Farnesyl pyrophosphate synthase (FPPS; EC 2.5.1.10) is a promising antibiotic drug target as it represents the point of convergence of these two pathways. The enzyme belongs to a large group of prenyltransferases responsible for the principal bond-forming reactions of isoprenoid biosynthesis. The mevalonate and nonmevalonate pathways both produce isopentenyl pyrophosphate (IPP), which along with its isomer dimethyl­allyl diphosphate (DMAPP) is converted through a ‘head-to-tail’ condensation reaction to form geranyl diphosphate (GPP) by FPPS. In summary, this work provides the first functional and structural insights into FPPS from the opportunistic pathogen P. aeruginosa.

Two structures of PaFPPS with bound GPP were determined in the course of this study: a ternary complex with GPP and Mg2+ and a quaternary complex with GPP, Mg2+ and a small molecule derived from screening of a fragment-based library. The overall structures of the enzyme sub­units in these two complexes are very similar to the structure of the unliganded enzyme (r.m.s.d. values of around 0.3 Å) and no large-scale conformational changes have been observed. Note that the lid region, residues Ala227–Gly254, is also disordered in these two structures. In the PaFPPS complex GPP is well defined in both subunits, whereas in the quaternary complex GPP is only bound to subunit A. However, the binding mode and interactions of GPP with protein residues and Mg2+ ions are identical in the two complexes. We were able to determine crystal structures of these hits with PaFPPS, including a ternary enzyme–GPP–SPB02696 complex. In the ternary PaFPPS–GPP–fragment complex, the fragments only bound to site SPB-1. Finally, we note a systematic difference in the occupancy of ligands in the two subunits of PaFPPS. It appears not to be related to soaking of ligands into the active site, i.e. differences in accessibility of the two active sites in the asymmetric unit, as this finding also holds for the PaFPPS–GPP–fragment complex obtained by co-crystallization. It is possible that these observations reflect cooperative behaviour in the dimeric enzyme with respect to substrate/ligand binding, but this remains to be corroborated by further experimental studies.

>[2x]SMIAAYQARCQARVDAALDALFVAPREELQRLYEAMRYSVMNGGKRVRPLLAYAACEALGGAPQRADAAACAVELIHAYSLVHDDLPAMDDDDLRRGQPTTHRAFDEATAILAADGLQALAFEVLADTRRNPQEHAVCLEMLTRLARAAGSAGMVGGQAIDLGSVGVALDQAALEVMHRHKTGALIEASVRLGALASGRAEPASLAALERYAEAIGLAFQVQDDILDVESDTATLGKTQGKDQAHNKPTYPALLGLEAAKGYALELRDLALAALDGFPPSADPLRQLARYIVERRN> MLPRKNLFSFTSKDPSAFGIHLAAAAREHSVYFDEGLGVPVVLRGADVVAVLRDSETFSTRTYDTGIMKGALVTLGGEAHTRMRRLFNAVLSPRVISRYEEATVTPVARRVVERLVRKERAELFDDFAISMPMGVTSALFGLPEERIAENDALIRKMIRSVVMPQDPVVVAEGRSAHAAME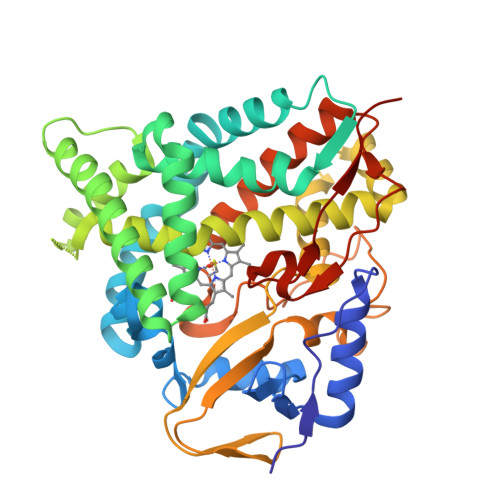AQLREIAEREVAHPSDTLLGEIARAIVAEGLGGVEACEGVVLTLILGSYETTSWMLANLLVALLAHPDAMNQLRQQPSLLPQAIEESTRWCSSAAGIVRFVEREATIGGETLAAGTILYLSLIARHYDEEIYPRPETFDIHRRPVGMLNFGGGLHYCVGAPLARMEARVGVSLLLERFPALRADPTVQPTFSTAPRGAAAFGPDQIPALLVHHHHHH>MAKKTSSKGKLPPGPLPLPGLGNLLHVDFQNTPYCFDQLRRRFGDVFSLQLAWTPVVVLNGLAAVREALVTHGEDTADRPPVPITQILGFGPRSQGVFLARYGPAWREQRRFSVSTLRNLGLGKKSLEQWVTEEAACLCAAFANHSGRPFRPNGLLDKAVSNVIASLTCGRRFEYDDPRFLRLLDLAQEGLKEESGFLREVLNAVPVLLHIPALAGKVLRFQKAFLTQLDELLTEHRMTWDPAQPPRDLTEAFLAEMEKAKGN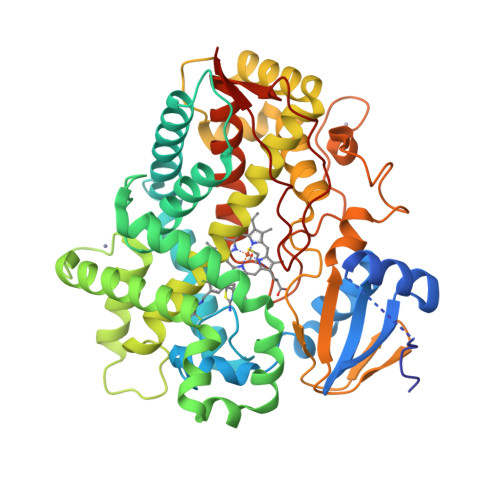PESSFNDENLRIVVADLFSAGMVTTSTTLAWGLLLMILHPDVQRRVQQEIDDVIGQVRRPEMGDQAHMPYTTAVIHEVQRFGDIVPLGVTHMTSRDIEVQGFRIPKGTTLITNLSSVLKDEAVWEKPFRFHPEHFLDAQGHFVKPEAFLPFSAGRRACLGEPLARMELFLFFTSLLQHFSFSVPTGQPRPSHHGVFAFLVSPSPYELCAVPRHHHH[4x]>[20x]MSVTTLGQSFPANAKVKYYYKLSEKQDLDAFVNSIFVGSYKLKQISYL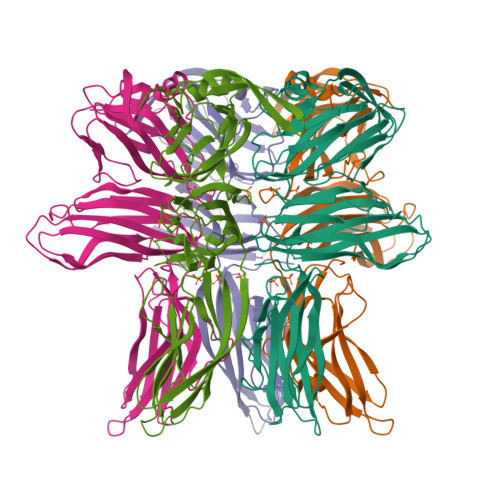LYGNTKIVSAPVVPLGPNASIIIDDELQEGLYLIRIKVYNTNSFSVTVTPFFNNNNTMTYSIGANSEFEIYDIFTKEQGNIYYIQLPPGLAILEFSLERVFEKGNRINIPKIIHTSGNGYISFRLRKGTYAIKMPYSYNNTTSTTFTNFQFGTISTSVATIPLVISSIPANGSGSGTFLVYLKITGDYEDVKFSVTYGGGLGVPFTFGLEVEEINELVENTNFVTQSVTLSGSQVTQSILNVQGSGSHLRLKYASVSGLTTAVTQCQLQATNLNRSTTYSTVWDFIAGGSSTPPSWDIREINSIQLVANGGSSTSSVTITLILVYEQIAGELSHHHHHH>[2x]MKKFLPGLLLMGLVACSSNQRMSDYSQPESQSDLAPKSSTTQFQPQPLLSKASSMPLNLL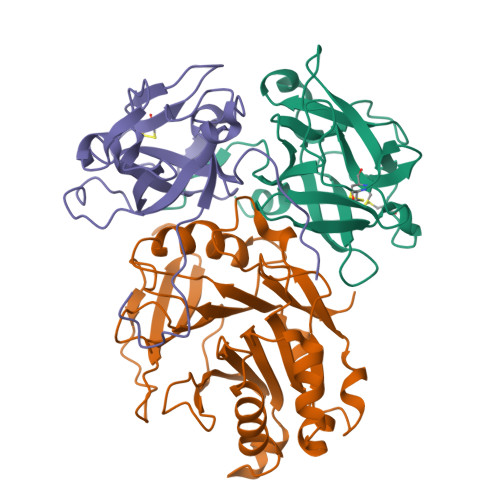SSSKNGQVSPSEPSNFMTLMGQNGALLTVWALAKRNWLWAYPNIYSQDFGNIRNWKIEPGKHREYFRFVNQSLGTCIEAYGNGLIHDTCSLDKLAQEFELLPTDSGAVVIKSVSQGRCVTYNPVSPTYYSTVTLSTCDGATEPLRDQTWYLAPPVLEATAVN;>[2x]MQWVKQLNVVFCTMLFSFSSYANLSDFKVATWNLQGSSAVNESKWNINVRQLLSGEQGADILMVQEAGSLPSSAVRTSRVIQHGGTPIEEYTWNLGTRSRPNMVYIYYSRLDVGANRVNLAIVSRRQADEAFIVHSDSSVLQSRPAVGIRIGTDVFFTVHALATGGSDAVSLIRNIFTTFTSSPSSPERRGYSWMVVGDFNRAPVNLEAALRQEPAVSENTIIIAPTEPTHRSGNILDYAILHDAHLPRREQARERIGASLMLNQLRSQITSDHFPVSFVHDR;>[2x]MKKYLLSFLLSMILTLTSHAESNPDPTTYPDVELSPPPRISLRSLLTAQPIKNDHYDSHNYLSTHWELIDYKGKEYEKLRDGGTLVQFKVVGAAKCFAFPGEGTTDCKDIDHTVFNLIPTNTGAFLIKDALLGFCMTSHDFDDLRLEPCGISVSGRTFSLAYQWGILPPFGPSKILRPPVGRNQGS2,6-DIMETHYL-1-(3-[3-METHYL-5-ISOXAZOLYL]-PROPANYL)-4-[2N-METHYL-2H-TETRAZOL-5-YL]-PHENOL | C17 H21 N5 O2 | 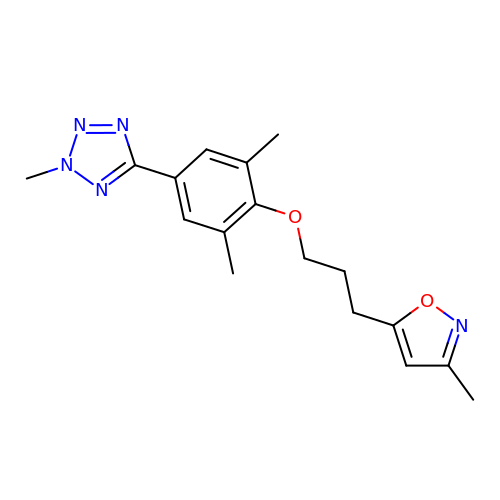RVZKQTQAFHEOKT-UHFFFAOYSA-N>MSLSSPNLSFYYNECERFESFLKNHHLHLESFHPYLEKAFFEMVLNGGKRFRPKLFLAVLCALVGQKDYS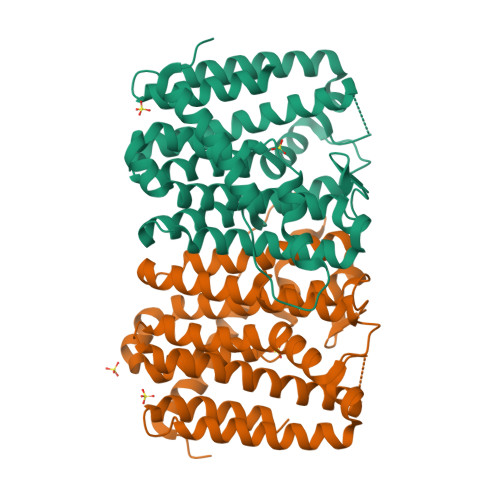NQQTEYFKIALSIECLHTYSLIHDDLPCMDNAALRRNHPTLHAKYDETTAVLIGDALNTYSFELLSNALLESHIIVELIKILSANGGIKGMILGQALDCYFENTPLNLEQLTFLHEHKTAKLISASLIMGLVASGIKDEELFKWLQAFGLKMGLCFQVLDDIIDVTQDEEESGKTTHLDSAKNSFVNLLGLERANNYAQTLKTEVLNDLDALKPAYPLLQENLNALLNTLFKGEGHHHHHH[4x]> CGAGACAACCAGGAGUCUAUAAAAUUCCCACUGAUGAGACUGGACGAAAGACAUGUAU;> ACAUGUCUCUGGGA

We have determined the crystal structure of a pseudoknot (PK)-containing hammerhead ribozyme that closely resembles the pistol ribozyme, with essentially identical secondary structure and connectivity. The core of the hammerhead ribozyme comprises a three-way helical junction containing largely conserved nucleotides of which G12 and G8 are functionally important. The structure is distinct from previously reported forms of hammerhead ribozyme structures in that it includes a pseudoknot in place of other tertiary contacts. Despite the similarity in overall structure to the pistol ribozyme, the local structure close to the cleavage site differs, and the PK hammerhead retains its unique mechanistic identity and demonstrates enhanced activity over other hammerhead ribozymes under standard conditions.

The ribozyme strand was synthesized by in vitro transcription by T7 RNA polymerase, while the substrate strand was chemically synthesized to include a 2’H substitution at the cytosine 5’ adjacent to the scissile phosphate to prevent cleavage during crystallization. The hybridized molecules crystallized in the hexagonal space group P6122. The pseudoknot (PK) is formed from a stem loop (we term helix IV), and is a 6 bp helix comprising four standard cis-Watson Crick base pairs, capped at either end by A:A and G:A cis-Watson Crick base pairs. The stem of the loop forming the PK helix (helix IV) comprises five Watson-Crick base pairs, but forms a minor-groove triplex interaction with the AUA4 sequence that connects helix IV to helix I. The phosphate backbone of the substrate strand forms a sharp turn close to 180° at the scissile phosphate, generating the ‘splayed apart’ conformation required to give an in-line attack geometry. The RNA that was crystalized lacked the 2’-hydroxyl group at C-1 (in order to prevent ribozyme cleavage), and we have therefore modeled this in place, switching the ribose pucker to C3’-endo conformation. The resulting conformation is close to perfect for in-line nucleophilic attack by the C-1 O2’, with an O2’ – P distance of 3.0 Å and a dihedral angle of 172.5°. The general base in the hammerhead ribozyme has been deduced to be G1225,27, and in the PK hammerhead ribozyme G12 N1 is 2.7 Å from the O2’ nucleophile in the cleavage reaction, so that it is well placed to remove the proton from the nucleophile. The O2’ of G8 has been proposed as the general acid in the extended hammerhead ribozyme, and the G8 O2’ is 2.9 Å from the O5’ leaving group in the PK hammerhead ribozyme, so that it is well positioned to donate a proton to the leaving group in the cleavage reaction. In the PK hammerhead ribozyme the base pairing of G8 directs its ribose towards the reaction center such that its O2’ is 2.9 Å from the O5’ with a C-O2’-O5’ angle of 102°, so the proton is directed towards the leaving group oxygen atom at close to the tetrahedral angle.>GSPEFDSLYPIAVLIDELRNEDVQLRLNSIKKLSTIALALGVERTRSELLPFLTDTIYDEDEVLLALAEQLGTFTTLVGGPEYVHCLLPPLESLATVEETVVRDKAVESLRAISHEHSPSDLEAHFVPLVKRLAGGDWFTSRTSACGLFSVCYPRVSSAVKAELRQYFRNLCSDDTPMVRRAAASKLGEFAKVLELDNVKSEIIPMFSNLASDEQDSVRLLAVEACVNIAQLLPQEDLEALVMPTLRQAAEDKSWRVRYMVADKFTELQKAVGPEITKTDLVPAFQNLMKDCEAEVRAAASHKVKEFCENLSADCRENVIMSQILPCIKELVSDANQHVKSALASVIMGLSPILGKDNTIEHLLPLFLAQLKDECPEVRLNIISNLDCVNEVIGIRQLSQSLLPAIVELAEDAKWRVRLAIIEYMPLLAGQ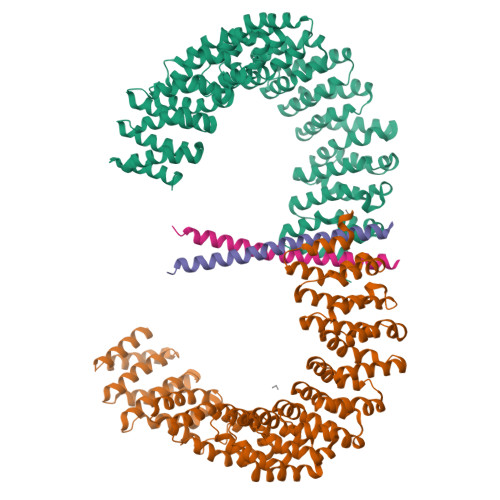LGVEFFDEKLNSLCMAWLVDHVYAIREAATSNLKKLVEKFGKEWAHATIIPKVLAMSGDPNYLHRMTTLFCINVLSEVCGQDITTKHMLPTVLRMAGDPVANVRFNVAKSLQKIGPILDNSTLQSEVKPILEKLTQDQDVDVKYFAQEALTVLSLA[4x];>STMDWEVERAELQARIAFLQGERKGQENLKKDLVRRIKMLEYALKQERAK[4x]> GPTGEAVERAIARVADTIGSGPVNSESIPALTAAETGHTSQVVPADTMQTRHVKNYHSRSESTVENFLCRSACVFYTTYRNHGTDGDNFGYWVISTRQV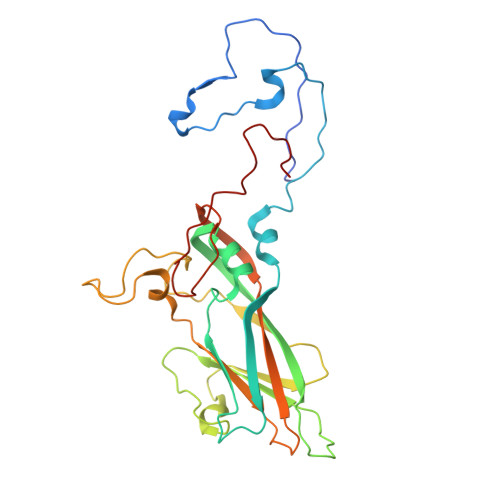AQLRRKLEMFTYARFDLELTFVITSTQEQSTIQGQDSPVLTHQIMYVPPGGPVPTKVNSYSWQTSTNPSVFWTEGSAPPRMSIPFISIGNAYSMFYDGWAKFDKQGTYGINTLNNMGTLYMRHVNDGSPGPIVSTVRIYFKPKHVKTWVPRPPRLCQYQKAGNVNFEPTGVTESRTDITTMQTT(2S)-4-(2-aminophenyl)-2-[(E)-({3-hydroxy-2-methyl-5-[(phosphonooxy)methyl]pyridin-4-yl}methylidene)amino]-4-oxobutanoic 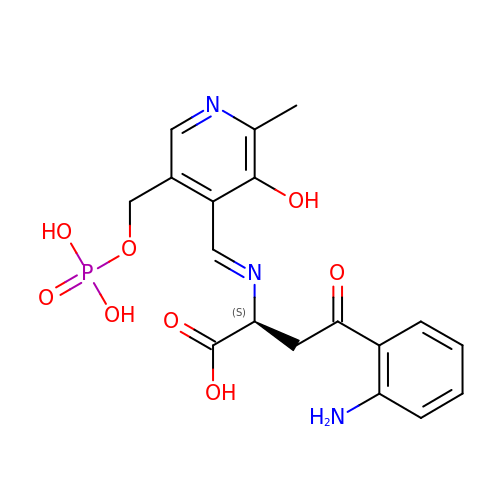acid | C18 H20 N3 O8 P | PUWQXAONJQUTHM-SJTXTDJHSA-N> VNNLYRELAPIPGPAWAEIEEEARRTFKRNIAGRRIVDVAGPTGFETSAVTTGHIRDVQSE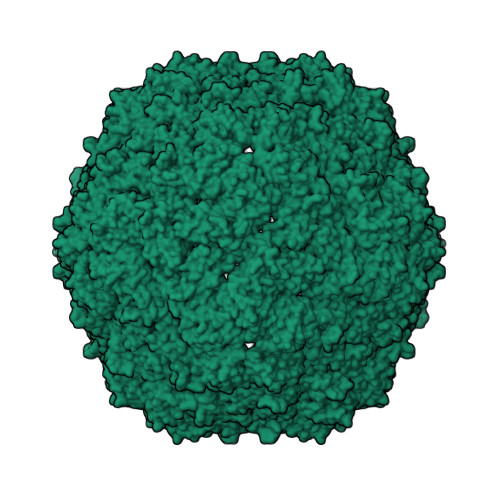TSGLQVKQRIVQEYIELRTPFTVTRQAIDDVARGSGDSDWQPVKDAATTIAMAEDRAILHGLDAAGIGGIVPGSSNAAVAIPDAVEDFADAVAQALSVLRTVGVDGPYSLLLSSAEYTKVSESTDHGYPIREHLSRQLGAGEIIWAPALEGALLVSTRGGDYELHLGQDLSIGYYSHDSETVELYLQETFGFLALTDESSVPLSL>GPLGSPEFLPLDERAFEKTLTPIIQEYFEHGDTNEVAEMLRDLNLGEMKSGVPVLAVSLALEGKASHREMTSKLLSDLCGTVMSTTDVEKSFDKL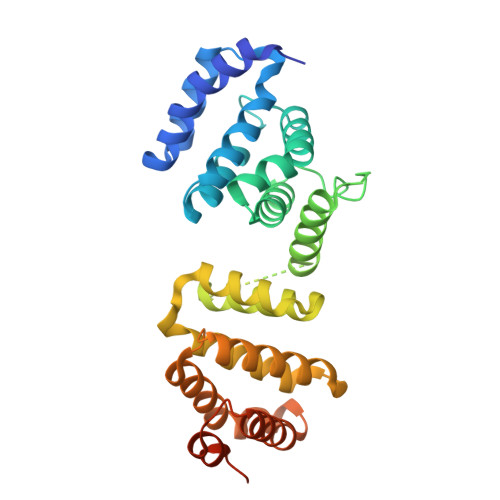LKDLPELALDTPRAPQLVGQFIARAVGDGILCNTYIDSYKGTVDCVQARAALDKATVLLSMSKGGKRKDSVWGSGGGQQSVNHLVKEIDMLLKEYLLSGDISEAEHCLKELEVPHFHHELVYEAIIMVLESTGESTFKMILDLLKSLWKSSTITVDQMKRGYERIYNEIPDINLDVPHSYSVLERFVEECFQAGIISKQLRDLCPSRGRKRFVSEGDGGRLKPESY[2x]> MEIVYKPLDIRNEEQFASIKKLIDADLSEPYSIYVYRYFLNQWPELTYIAVDNKSGTPNIPIGCIVCKMDPHRNVRLRGYIGMLAVESTYRGHGIAKKLVEIAIDKMQREHCDEIMLETEVENSAALNLYEGMGFIRMKRMFRYYLNEGDAFKLILPLT;> GPMEVDSILGSLSITDDFDQLVDVTSLFDELCSKLKPEAIVKDPRFDLFEGTHSLEVNNSKLDSSLIELTAEEIEFDVNVAYDPPLASVAAIADRLLRCVISWLNDYQTLPTTVLSCRYTESLLSSLVKGTT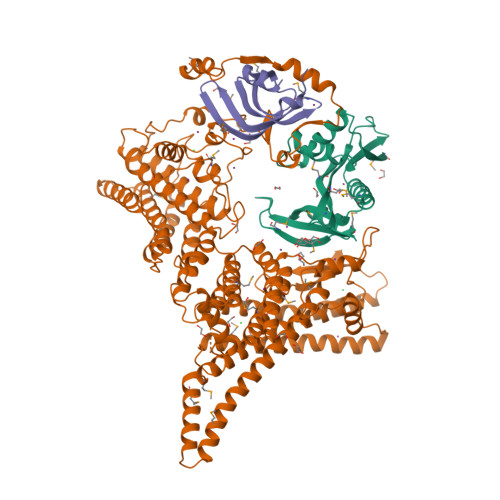AGSSWCTGNILYDKVLGSCILGVCYLTKFVQKLLSAGIVFEEEDLNFNNMGFNTFDNLPGQDVVINSLTESLQILEAYSDDSLHLTMLKHILKIIICLVHLEDHLTDYSTKTSHLDELIENANSVNGIFPQLQLSPPKGAFSTYIQKHRSNQFPPRKITKLPTDYSGFITLANDVKTILLVDKAESALETYQFAKFFNKLEQRHVIARILFPLFFIRDDRTVLGKFSYTQFYLLHVKEFSAQTPSEFESSIGNELIQESSNMLLEWYQNCSQNTCRYRQGFNRQLILWDSLQAQFESVNSQVYCSWTYFMKLSSMIEFSLKGFDLDIYKPFEAYSMFWYVYYLSHHLETFLKDSQNDIESNINAIHSMNKKLKKLKAGEKKDQLRLKYRFAMDNEMEQLQATKQFLNYLLKEINITKSLCLIEVFQFAILKSFGLIDNKNSTPSKFSNERLIHNLRFKPFNSIGVPELPEYEVFQQTLKDFVIEEKGAAFDIKLERATNFIETEVRNVVSSIDEIMQGIKGGDNNGVLVTGTRLVQELSLEYYCKLKHTSKALSVNSKVIVNTLKKNIKNKDSHEYKVELVHTTEGWNYFPIQTLRIKQDRYK;> MDILKLSDFIGNTLIVSLTEDRILVGSLVAVDAQMNLLLDHVEERMGSSSRMMGLVSVPRRSVKTIMIDKPVLQELT3-(2~{H}-indazol-3-yl)-~{N}-[[1-[(1~{R},2~{R})-2-methoxycyclohexyl]-1,2,3-triazol-4-yl]methyl]-5-(propanoylamino)benzamide 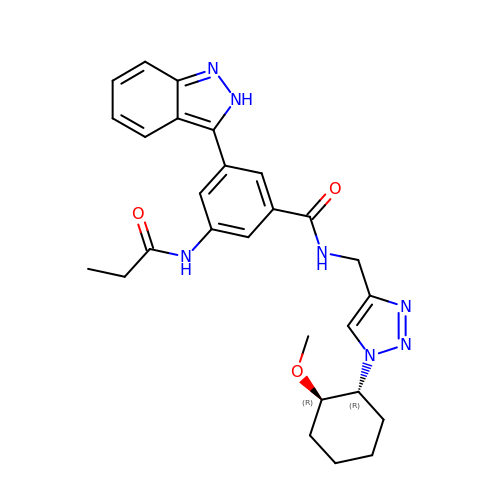| C27 H31 N7 O3 | SQKSGNQRUQLTDE-DNQXCXABSA-N>[3x]FFTCNSNANLSMLQLGVPDNSSTIVTGLLPTHWFCANQSTSVYSANGFFYIDVGNHRSAFALHTGYYDANQYYIYVTNEIGLNASVTLKICKFSRNTTFDFLSNASSSFDCIVNLLFTEQLGAPLGITISGETVRLHLYNVTRTFYVPAAYKLTKLSVKCYFNYSCVFSVVNATVTVNVTTHNGRVVNYTVCDDCNGYTDNIFSVQQDGRIPNGFPFNNWFLLTNGSTLVDGVSRLYQPLRLTCLWPVPGLKSSTGFVYFNATGSDVNCNGYQHNSVVDVMRYNLNFSANSLDNLKSGVIVFKTLQYDVLFYCSNSSSGVLDTTIPFGPSSQPYYCFINSTINTTHVSTFVGILPPTVREIVVARTGQFYINGFKYFDLGFIEAVNFNVTTASATDFWTVAFATFVDVLVNVSATNIQNLLYCDSPFEKLQCEHLQFGLQDGFYSANFLDDNVLPETYVALPIYYQHTDINFTATASFGGSCYVCKPHQVNISLNGNTSVCVRTSHFSIRYIYNRVKSGSPGDSSWHIYLKSGTCPFSFSKLNNFQKFKTICFSTVEVPGSCNFPLEATWHYTSYTIVGALYVTWSEGNSITGVPYPVSGIREFSNLVLNNCTKYNIYDYVGTGIIRSSNQSLAGGITYVSNSGNLLGFKNVSTGNIFIVTPCNQPDQVAVYQQSIIGAMTAVNESRYGLQNLLQLPNFYYVSNGGNNCTTAVMTYSNFGICADGSLIPVRPRNSSDNGISAIITANLSIPSNWTTSVQVEYLQITSTPIVVDCATYVCNGNPRCKNLLKQYTSACKTIEDALRLSAHLETNDVSSMLTFDSNAFSLANVTSFGDYNLSSVLPQRNIRSSRIAGRSALEDLLFSKVVTSGLGTVDVDYKSCTKGLSIADLACAQYYNGIMVLPGVADAERMAMYTGSLIGGMVLGGLTSAAAIPFSLALQARLNYVALQTDVLQE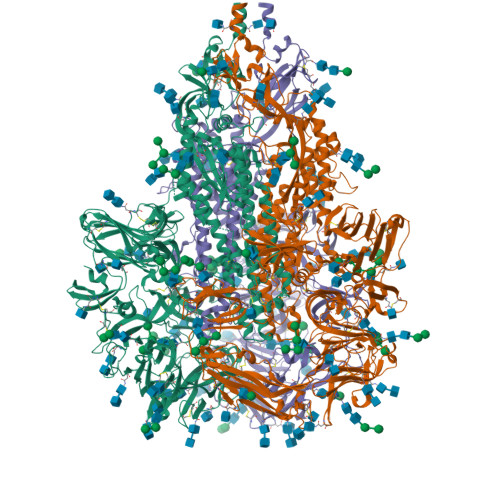NQKILAASFNKAINNIVASFSSVNDAITQTAEAIHTVTIALNKIQDVVNQQGSALNHLTSQLRHNFQAISNSIQAIYDRLDSIQADQQVDRLITGRLAALNAFVSQVLNKYTEVRGSRRLAQQKINECVKSQSNRYGFCGNGTHIFSIVNSAPDGLLFLHTVLLPTDYKNVKAWSGICVDGIYGYVLRQPNLVLYSDNGVFRVTSRVMFQPRLPVLSDFVQIYNCNVTFVNISRVELHTVIPDYVDVNKTLQEFAQNLPKYVKPNFDLTPFNLTYLNLSSELKQLEAKTASLFQTTVELQGLIDQINSTYVDLKLLNRFENLIKRMKQIEDKIEEIESKQKKIENEIARIKKIKLVPRGSLEWSHPQFEK> QPAQTIPWGIERVKAPSVWSITDGSVSVIQVAVLDTGVDYDHPDLAANIAWCVSTLRGKVSTKLRDCADQNGHGTHVIGTIAALNNDIGVVGVAPGVQIYSVRVLDARGSGSYSDIAIGIEQAILGPDGVADKDGDGIIAGDPDDDAAEVISMSLGGPADDSYLYDMIIQAYNAGIVIVAASGNEGAPSPSYPA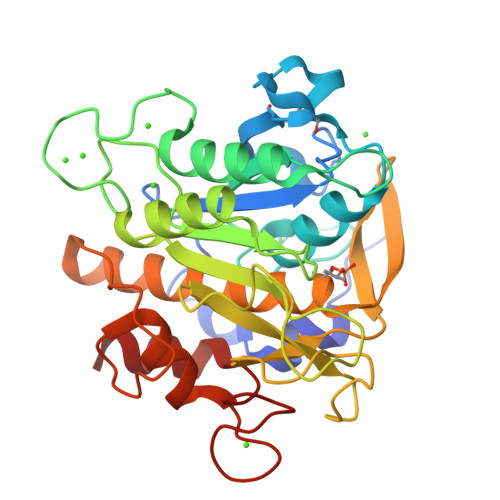AYPEVIAVGAIDSNDNIASFSNRQPEVSAPGVDILSTYPDDSYETLMGTSMATPHVSGVVALIQAAYYQKYGKILPVGTFDDISKNTVRGILHITADDLGPTGWDADYGYGVVRAALAVQAALG>[6x]MAAPARDPPGYRYAAAMVPTGSILSTIEVASHRRLFDFFAAVRSDENSLYDVEFDALLGSYCNTLSLVRFLELGLSVACVCTKFPELAYMNEGRVQFEVHQPLIARDGPHPVEQPVHNYMTKVIDRRALNAAFSLATEAIALLTGEALDGTGISLHRQLRAIQQLARNVQAVLGAFERGTADQMLHVLLEKAPPLALLLPMQRYLDNGRLATRVARATLVAELKRSFCDTSFFLGKAGHRREAIEAWLVDLTTATQPSVAVPRLTHADTRGRPVDGVLVTTAAIKQRLLQSFLKVEDTEADVPVTYGEMVLNGANLVTALVMGKAVRSLDDVGRHLLDMQEEQLEANRETLDELESAPQTTRVRADLVAIGDRLVFLEALEKRIYAATNVPYPLVGAMDLTFVLPLGLFNPAMERFAAHAGDLVPAPGHPEPRAFPPRQLFFWGKDHQVLRLSMENAVGTVCHPSLMNIDAAVGGVNHDPVEAANPYGAYVAAPAGPGADMQQRFLNAWRQRLAHGRVRWVAECQMTAEQFMQPDNANLALELHPAFDFFAGVADVELPGGEVPPAGPGAIQATWRVVNGNLPLALCPVAFRDARGLELGVGRHAMAPATIAAVRGAFEDRSYPAVFYLLQAAIHGNEHVFCALARLVTQCITSYWNNTRCAAFVNDYSLVSYIVTYLGGDLPEECMAVYRDLVAHVEALAQLVDDFTLPGPELGGQAQAELNHLMRDPALLPPLVWDCDGLMRHAALDRHRDCRIDAGGHEPVYAAACNVATADFNRNDGRLLHNTQARAADAADDRPHRPADWTVHHKIYYYVLVPAFSRGRCCTAGVRFDRVYATLQNMVVPEIAPGEECPSDPVTDPAHPLHPANLVANTVKRMFHNGRVVVDGPAMLTLQVLAHNMAERTTALLCSAAPDAGANTASTANMRIFDGALHAGVLLMAPQHLDHTIQNGEYFYVLPVHALFAGADHVANAPNFPPALRDLARHVPLVPPALGANYFSSIRQPVVQHARESAAGENALTYALMAGYFKMSPVALYHQLKTGLHPGFGFTVVRQDRFVTENVLFSERASEAYFLGQLQVARHETGGGVNFTLTQPRGNVDLGVGYTAVAATGTVRNPVTDMGNLPQNFYLGRGAPPLLDNAAAVYLRNAVVAGNRLGPAQPLPVFGCAQVPRRAGMDHGQDAVCEFIATPVATDINYFRRPCNPRGRAAGGVYAGDKEGDVIALMYDHGQSDPARPFAATANPWASQRFSYGDLLYNGAYHLNGASPVLSPCFKFFTAADITAKHRCLERLIVETGSAVSTATAASDVQFKRPPGCRELVEDPCGLFQEAYPITCASDPALLRSARDGEAHARETHFTQYLIYDASPLKGLSL;>[6x]MAAPQFHRPSTITADNVRALGTRGLVLATNNAQFIMDNSYPHPHGTQGAVREFLRGQAAALTDLGVTHANNTFAPQPMFAGDAAAEWLRPSFGLKRTYSPFVVRDPKTPSTP;>MITDCFEADIAIPSGISRPDAAALQRCEGRVVFLPTIRRQLALADVAHESFVSGGVSPDTLGLLLAYRRRFPAVITRVLPTRIVACPVDLGLTHAGTVNLRNTSPVDLCNGDPVSLVPPVFEGQATDVRLESLDLTLRFPVPLPTPLAREIVARLVARGIRDLNPDPRTPGELPDLNVLYYNGARLSLVADVQQLASVNTELRSLVLNMVYSITEGTTLILTLIPRLLALSAQDGYVNALLQMQSVTREAAQLIHPEAPMLMQDGERRLPLYEALVAWLAHAGQLGDILALAPAVRVCTFDGAAVVQSGDMAPVIRYP[2x];> MKTKPLPTAPMAWAESAVETTTSPRELAGHAPLRRVLRPPIARRDGPVLLGDRAPRRTASTMWLLGIDPAESSPGTRATRDDTEQAVDKILRGARRAGGLTVPGAPRYHLTRQVTLTDLCQPNAERAGALLLALRHPTDLPHLARHRAPPGRQTERLAEAWGQLLEASALGSGRAESGCARAGLVSFNFLVAACAAAYDARDAAEAVRAHITTNYGGTRAGARLDRFSECLRAMVHTHVFPHEVMRFFGGLVSWVTQDELASVTAVCSGPQEATHTGHPGRPRSAVTIPACAFVDLDAELCLGGPGAAFLYLVFTYRQCRDQELCCVYVVKSQLPPRGLEAALERLFGRLRITNTIHGAEDMTPPPPNRNVDFPLAVLAASSQSPRCSASQVTNPQFVDRLYRWQPDLRGRPTARTCTYAAFAELGVMPDDSPRCLHRTERFGAVGVPVVILEGVVWRPGGWRACA;> MNAHFANEVQYDLTRDPSSPASLIHVIISSECLAAAGVPLSALVRGRPDGGAAANFRVETQTRAHATGDCTPWRSAFAAYVPADAVGAILAPVIPAHPDLLPRVPSAGGLFVSLPVACDAQGVYDPYTVAALRLAWGPWATCARVLLFSYDELVPPNTRYAADGARLMRLCRHFCRYVARLGAAAPAAATEAAAHLSLGMGESGTPTPQASSVSGGAGPAVVGTPDPPISPEEQLTAPGGDTATAEDVSITQENEEILALVQRAVQDVTRRHPVRARPKHAASGVASGLRQGALVHQAVSGGALGASDAEAVLAGLEPPGGGRFASRGGPRAAGEDVLNDVLTLVPGTAKPRSLVEWLDRGWEALAGGDRPDWLWSRRSISVVLRHHYGTKQRFVVVSYENSVAWGGRRARPPRLSSELATALTEACAAERVVRPHQLSPAAQTALLRRFPALEGPLRHPRPVLQPFDIAAEVAFVARIQIACLRALGHSIRAALQGGPRIFQRLRYDFGPHQSEWLGEVTRRFPVLLENLMRALEGTAPDAFFHTAYALAVLAHLGGQGGRGRRRRLVPLSDDIPARFADSDAHYAFDYYSTSGDTLRLTNRPIAVVIDGDVNGREQSKCRFMEGSPSTAPHRVCEQYLPGESYAYLCLGFNRRLCGLVVFPGGFAFTINTAAYLSLADPVARAVGLRFCRGAATGPGLVR;>[2x]MDPYYPFDALDVWEHRRFIVADSRSFITPEFPRDFWMLPVFNIPRETAAERAAVLQAQRTAAAAALENAALQAAELPVDIERRIRPIEQQVHHIADALEALETAAAAAEEADAARDAEARGEGAADGAAPSPTAGPAAAEMEVQIVRNDPPLRYDTNLPVDLLHMVYAGRGAAGSSGVVFGTWYRTIQERTIADFPLTTRSADFRDGRMSKTFMTALVLSLQSCGRLYVGQRHYSAFECAVLCLYLLYRTTHESSPDRDRAPVAFGDLLARLPRYLARLAAVIGDESGRPQYRYRDDKLPKAQFAAAGGRYEHGALATHVVIATLVRHGVLPAAPGDVPRDTSTRVNPDDVAHRDDVNRAAAAFLARGHNLFLWEDQTLLRATANTITALAVLRRLLANGNVYADRLDNRLQLGMLIPGAVPAEAIARGASGLDSGAIKSGDNNLEALCVNYVLPLYQADPTVELTQLFPGLAALCLDAQAGRPLASTRRVVDMSSGARQAALVRLTALELINRTRTNTTPVGEIINAHDALGIQYEQGPGLLAQQARIGLASNTKRFATFNVGSDYDLLYFLCLGFIPQYLSVA;>MIPAALPHPTMKRQGDRDIVVTGVRNQFATDLEPGGSVSCMRSSLSFLSLLFDVGPRDVLSAEAIEGCLVEGGEWTRAAAGSGPPRMCSIIELPNFLEYPAARGGLRCVFSRVYGEVGFFGEPTAGLLETQCPAHTFFAGPWAMRPLSYTLLTIGPLGMGLYRDGDTAYLFDPHGLPAGTPAFIAKVRAGDVYPYLTYYAHDRPKVRWAGAMVFFVPSGPGAVAPADLTAAALHLYGASETYLQDEPFVERRVAITHPLRGEIGGLGALFVGVVPRGDGEGSGPVVPALPAPTHVQTPGADRPPEAPRGASGPPDTPQAGHPNRPPDDVWAAALEGTPPAKPSAPDAAASGPPHAAPPPQTPAGDAAEEAEDLRVLEVGAVPVGRHRARYSTGLPKRRRPTWTPPSSVEDLTSGERPAPKAPPAKAKKKSAPKKKAPVAAEVPASSPTPIAATVPPAPDTPPQSGQGGGDDGPASPSSPSVLETLGARRPPEPPGADLAQLFEVHPNVAATAVRLAARDAALAREVAACSQLTINALRSPYPAHPGLLELCVIFFFERVLAFLIENGARTHTQAGVAGPAAALLDFTLRMLPRKTAVGDFLASTRMSLADVAAHRPLIQHVLDENSQIGRLALAKLVLVARDVIRETDAFYGDLADLDLQLRAAPPANLYARLGEWLLERSRAHPNTLFAPATPTHPEPLLHRIQALAQFARGEEMRVEAEAREMREALDALARGVDSVSQRAGPLTVMPVPAAPGAGGRAPCPPALGPEAIQARLEDVRIQARRAIESAVKEYFHRGAVYSAKALQASDSHDCRFHVASAAVVPMVQLLESLPAFDQHTRDVAQRAALPPPPPLATSPQAILLRDLLQRGQPLDAPEDLAAWLSVLTDAATQGLIERKPLEELARSIHGINDQQARRSSGLAELQRFDALDAALAQQLDSDAAFVPATGPAPYVDGGGLSPEATRMAEDALRQARAMEAAKMTAELAPEARSRLRERAHALEAMLNDARERAKVAHDAREKFLHKLQGVLRPLPDFVGLKACPAVLATLRASLPAGWTDLADAVRGPPPEVTAALRADLWGLLGQYREALEHPTPDTATALAGLHPAFVVVLKTLFADAPETPVLVQFFSDHAPTIAKAVSNAINAGSAAVATASPAATVDAAVRAHGALADAVSALGAAARDPASPLSFLAVLADSAAGYVKATRLALEARGAIDELTTLGSAAADLVVQARRACAQPEGDHAALIDAAARATTAARESLAGHEAGFGGLLHAEGTAGDHSPSGRALQELGKVIGATRRRADELEAAVADLTAKMAAQRARGSSERWAAGVEAALDRVENRAEFDVVELRRLQALAGTHGYNPRDFRKRAEQALAANAEAVTLALDTAFAFNPYTPENQRHPMLPPLAAIHRLGWSAAFHAAAETYADMFRVDAEPLARLLRIAEGLLEMAQAGDGFIDYHEAVGRLADDMTSVPGLRRYVPFFQHGYADYVELRDRLDAIRADVHRALGGVPLDLAAAAEQISAARNDPEATAELVRTGVTLPCPSEDALVACAAALERVDQSPVKNTAYAEYVAFVTRQDTAETKDAVVRAKQQRAEATERVMAGLREALAARERRAQIEAEGLANLKTMLKVVAVPATVAKTLDQARSVAEIADQVEVLLDQTEKTRELDVPAVIWLEHAQRTFETHPLSAARGDGPGPLARHAGRLGALFDTRRRVDALRRSLEEAEAEWDEVWGRFGRVRGGAWKSPEGFRAMHEQLRALQDTTNTVSGLRAQPAYERLSARYQGVLGAKGAERAEAVEELGARVTKHTALCARLRDEVVRRVPWEMNFDALGGLLAEFDAAAADLAPWAVEEFRGARELIQYRMGLYSAYARAGGQTGAGAESAPAPLLVDLRALDARARASSSPEGHEVDPQLLRRRGEAYLRAGGDPGPLVLREAVSALDLPFATSFLAPDGTPLQYALCFPAVTDKLGALLMRPEAACVRPPLPTDVLESAPTVTAMYVLTVVNRLQLALSDAQAANFQLFGRFVRHRQATWGASMDAAAELYVALVATTLTREFGCRWAQLGWASGAAAPRPPPGPRGSQRHCVAFNENDVLVALVAGVPEHIYNFWRLDLVRQHEYMHLTLERAFEDAAESMLFVQRLTPHPDARIRVLPTFLDGGPPTRGLLFGTRLADWRRGKLSETDPLAPWRSALELGTQRRDVPALGKLSPAQALAAVSVLGRMCLPSAALAALWTCMFPDDYTEYDSFDALLAARLESGQTLGPAGGREASLPEAPHALYRPTGQHVAVLAAATHRTPAARVTAMDLVLAAVLLGAPVVVALRNTTAFSRESELELCLTLFDSRPGGPDAALRDVVSSDIETWAVGLLHTDLNPIENACLAAQLPRLSALIAERPLADGPPCLVLVDISMTPVAVLWEAPEPPGPPDVRFVGSEATEELPFVATAGDVLAASAADADPFFARAILGRPFDASLLTGELFPGHPVYQRPLADEAGPSAPTAARDPRDLAGGDGGSGPEDPAAPPARQADPGVLAPTLLTDATTGEPVPPRMWAWIHGLEELASDDAGGPTPNPAPALLPPPATDQSVPTSQYAPRPIGPAATARETRPSVPPQQNTGRVPVAPRDDPRPSPPTPSPPADAALPPPAFSGSAAAFSAAVPRVRRSRRTRAKSRAPRASAPPEGWRPPALPAPVAPVAASARPPDQPPTPESAPPAWVSALPLPPGPASARGAFPAPTLAPIPPPPAEGAVVPGGDRRRGRRQTTAGPSPTPPRGPAAGPPRRLTRPAVASLSASLNSLPSPRDPADHAAAVSAAAAAVPPSPGLAPPTSAVQTSPPPLAPGPVAPSEPLCGWVVPGGPVARRPPPQSPATKPAARTRIRARSVPQPPLPQPPLPQPPLPQPPLPQPPLPQPPLPQPPLPQPPLPQPPLPQPPLPQPPLPPVTRTLTPQSRDSVPTPESPTHTNTHLPVSAVTSWASSLALHVDSAPPPASLLQTLHISSDDEHSDADSLRFSDSDDTEALDPLPPEPHLPPADEPPGPLAADHLQSPHSQFGPLPVQANAVLSRRYVRSTGRSALAVLIRACRRIQQQLQRTRRALFQRSNAVLTSLHHVRMLLG[2x]

Here we show asymmetric reconstructions of herpes simplex virus 2 (HSV-2) B- (containing scaffold proteins inside, putative capsid assembly intermediate), C- (DNA-filled capsid, derived from the enveloped virion by using detergent treatment to remove viral membrane proteins and outer tegument proteins) and virion-capsids (enveloped intact virion) at 8.1, 9.0 and 10.2 Å respectively. The asymmetric reconstructions reveal a unique portal vertex in the context of the icosahedral capsid, including 1 portal, 11 pentons, 3 types of hexons (P, peripentonal; E, edge; C, center) with the hexameric rings formed by VP26s, 320 triplexes (Ta-Tf) and 12 pentagram-shaped capsid vertex specific component (CVSC) densities (composed of a UL17 monomer, a UL25 dimer and a UL36 dimer, presence in C- and virion-capsids). Radially colored representations of the three reconstructions reveal the dodecameric portal situated beneath one of the pentameric vertices; but, the density surrounding the portal displays a five-fold symmetrical assembly, highlighting the symmetry-mismatch structural features. The portal vertex of the capsid is a hub for protein-protein interactions that are important for capsid assembly and genome packaging.

When five-fold symmetry was imposed, the resolution of local reconstructions for the portal vertex in B-, C- and virion-capsids was improved to 4.05, 4.50 and 5.36 Å, respectively, albeit that the portal was five-fold averaged. The resulting density maps clearly reveal the polypeptide backbone, many bulky side chains, and atomic models of the portal vertex associated P-hexon (PVP-Hex), Ta and PVAT (not in B-capsid) from three capsids were built. Despite distinct organizations of the CVSC at the portal and penton vertices, the packaged dsDNA is visible in the C- and virion-capsids. In contrast to B-capsid, small tail-like density, previously named Portal Vertex Associated Tegument (PVAT), extends outwards from the portal vertex in the C- and virion-capsids, suggesting a possible role in genome retention and release. A comparison of asymmetric reconstructions of the portal vertex of the three capsids reveals notable differences in the position and morphology of the portal and PVAT. In contrast, five 10-nm-long coiled coils in the virion-capsid exhibit altered configurations to the counterparts in B-capsid to recruit the PVAT layers (UL25 C-domain), ensuring the retention of DNA. Interestingly a novel network of subunit contacts is observed between the portal and PV-Ta and varies each other in three capsids. Lying on the portal head, a novel five-fold symmetrical assembly comprising five copies of a well-resolved two-helix coiled coil (presumably being the fragment from the portal or pUL36) shows close contacts with PV-Ta.> DYSNPGHHPP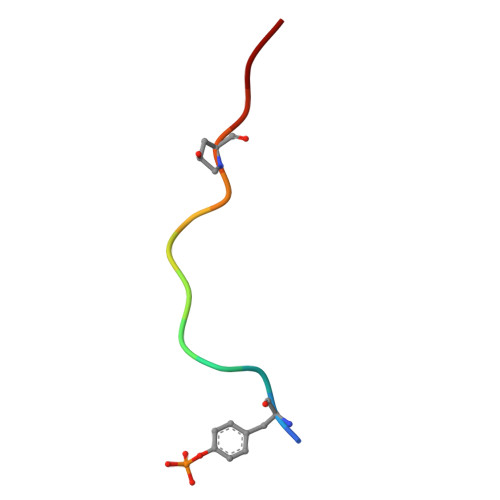RHN> MGRFIFVSFGLLVVFLSLSGTGADCPSGWSSYEGHCYKPFNEPKNWADAERFCKLQPKHSHLVSFQSAEEADFVVKLTRPRLKANLVWMGLSNIWHGCNWQWSDGARLN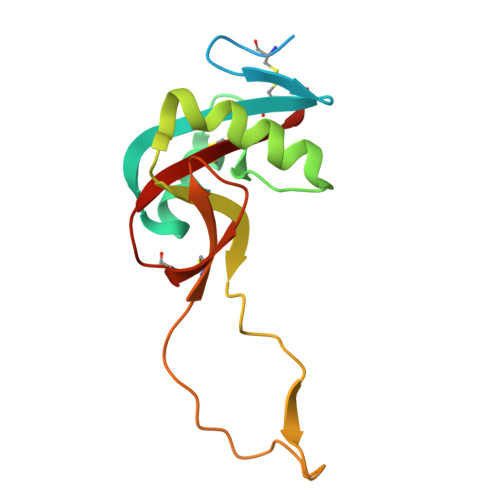YKDWQEQSECLAFRGVHTEWLNMDCSSTCSFVCKFKA> MSAEVIHQVEEALDTDEKEMLLFLCRDVAIDVVPPNVRDLLDILRERGKLSVGDLAELLYRVRRFDLLKRILKMDRKAVETHLLRNPHLVSDYRVLMAEIGEDLDKSDVSSLIFLMKDYMGRG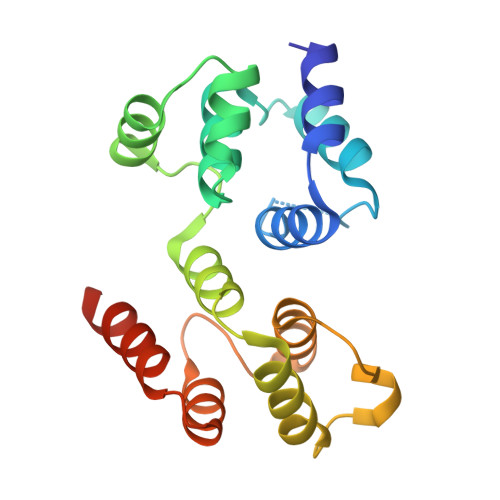KISKEKSFLDLVVELEKLNLVAPDQLDLLEKCLKNIHRIDLKTKIQKYKQSVQGAGTS> SGIVQQQNDLLRAIEAQQHLLQLTVWGIKQLQARSGGRGGWMEWDREINNYTSLIHSLIEESQN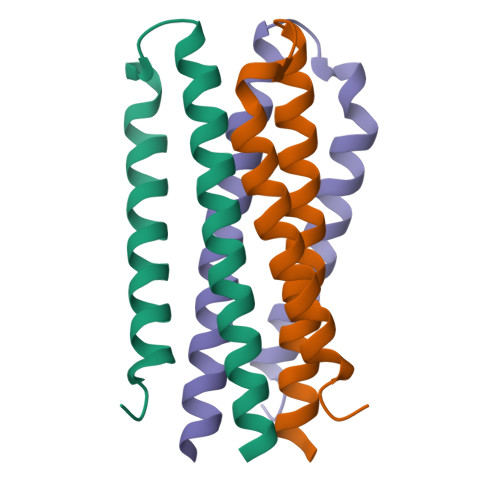QQEK>[2x]MERPQPDSMPQDLSEALKEATKEVHTQAENAEFMRNFQKGQVTRDGFKLVMASLYH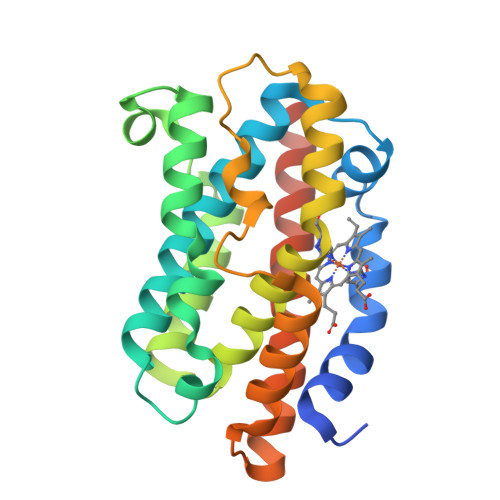IYVALEEEIERNKESPVFAPVYFPEELHRKAALEQDLAFWYGPRWQEVIPYTPAMQRYVKRLHEVGRTEPELLVAHAYTRYLGDLSHGQVLKKIAQKALDLPSSGEGLAFFTFPNIASATKFKQLYESRMNSLEMTPAVRQRVIEEAKTAFLLNIQLFEELQELLTHDTKDQSPSRA> GVALGATRVIYPAGQKQEQLAVTNNDENSTYLIQSWVENADGVKDGRF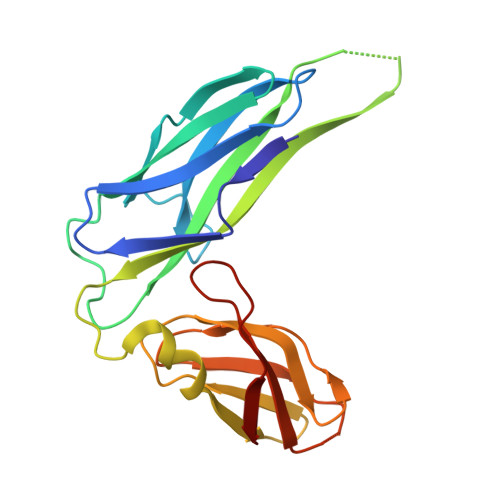IVTPPLFAMKGKKENTLRILDATNNQLPQDRESLFWMNVKAIPSMDKSKLTENTLQLAIISRIKLYYRPAKLALPPDQAAEKLRFRRSANSLTLINPTPYYLTVTELNAGTRVLENALVPPMGESTVKLPSDAGSNITYRTINDYGALTPKMTGVME> MSNYPLHQACMENEFFKVQELLHSKPSLLLQKDQDGRIPLHWSVSFQAHEITSFLLSKMENVNLDDYPDDSGWTPFHIACSVGNLEVVKSLYDRPLKPDLNKITNQGVTCLHLAVGKKWFEVSQFLIENGASVRIKDKFNQIPLHRAASVGSLKLIELLCGLGKSAVNWQDKQGWTPLFHALAEGHGDAAVLLVEKYGAEYDLVDN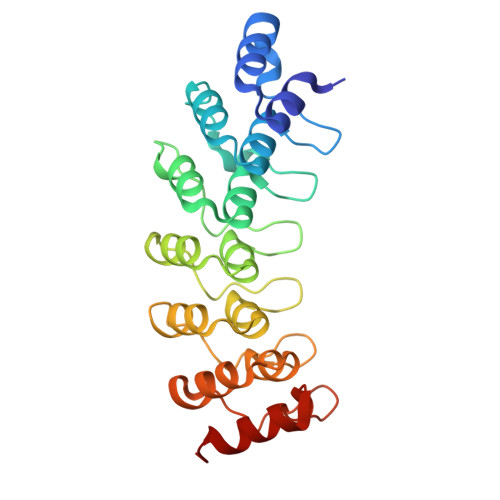KGAKAEDVALNEQVKKFFLNNVVDA>[7x]MSETREARISRAKRAFVSTPSVRKILSYMDRCRDLSDLESEPTCMMVYGASGVGKTTVIKKYLNQNRRESEAGGDIIPVL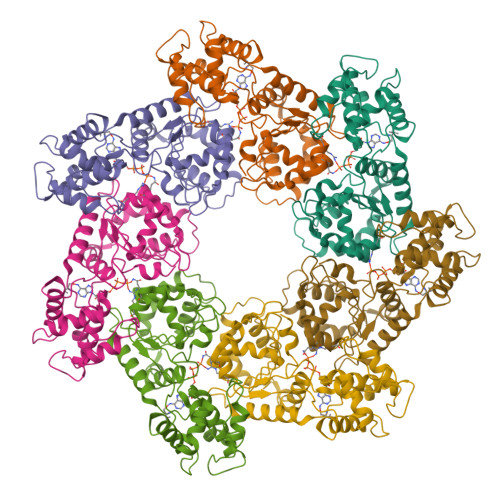HIELPDNAKPVDAARELLVEMGDPLALYETDLARLTKRLTELIPAVGVKLIIIDEFQHLVEERSNRVLTQVGNWLKMILNKTKCPIVIFGMPYSKVVLQANSQLHGRFSIQVELRPFSYNGGRGVFKTFLEYLDKALPFEKQAGLANESLQKKLYAFSQGNMRSLRNLIYQASIEAIDNQHETITEEDFVFASKLTSGDKPNSWKNPFEEGVEVTEDMLRPPPKDIGWEDYLRHSTPRVSKPGRNKNFFE2-amino-8-[trans-4-(2-hydroxyethoxy)cyclohexyl]-6-(6-methoxypyridin-3-yl)-4-methylpyrido[2,3-d]pyrimidin-7(8H)-one 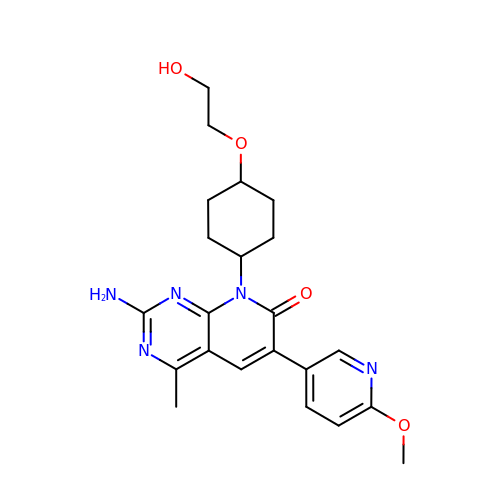| C22 H27 N5 O4 | XDLYKKIQACFMJG-WKILWMFISA-N> AMADIGSEFGHRTLASTPALWASIPCPRSELRLDLVLPSGQSFRWREQSPAHWSGVLADQVWTLTQTEEQLHCTVYRGDKS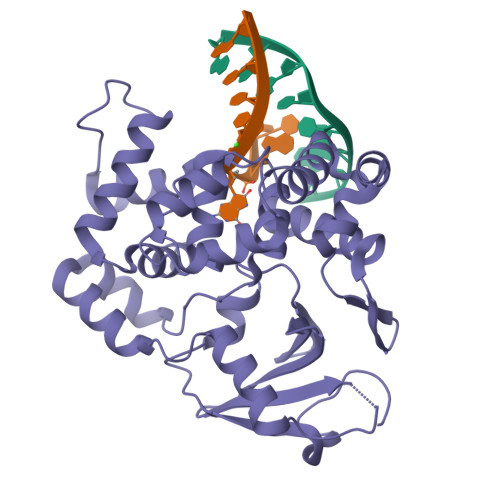QASRPTPDELEAVRKYFQLDVTLAQLYHHWGSVDSHFQEVAQKFQGVRLLRQDPIECLFSFICSSCNNIARITGMVERLCQAFGPRLIQLDDVTYHGFPSLQALAGPEVEAHLRKLGLGYRARYVSASARAILEEQGGLAWLQQLRESSYEEAHKALCILPGVGTKVADCICLMALDKPQAVPVDVHMWHIAQRDYSWHPTTSQAKGPSPQTNKELGNFFRSLWGPYAGWAFAVLFSADLRQSR>[3x]AGSFVEMVDNLRGKSGQGYYVEMTVGSPPQTLNILVDTGSSNFAVGAAPHPFLHRYYQRQLSSTYRDLRKGVYVPYTQGKWEGELGTDLVSIPHGPNVTVRANIAAITESDKFFINGSNWEGILGLAYAEIARPDDSLEPFFDSLVKQTHVPNLFSLQLCGAGFPLNQSEVLASVGGSMIIGGIDHSLYTG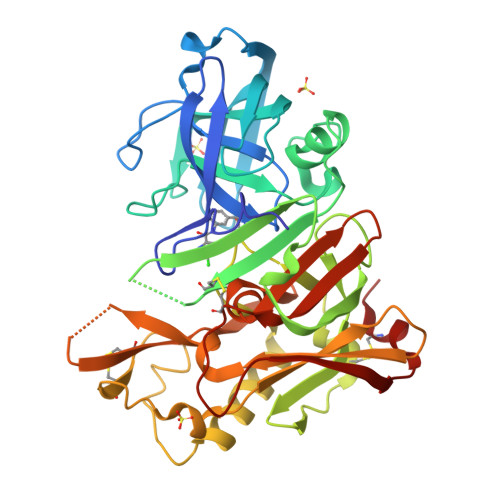SLWYTPIRREWYYEVIIVRVEINGQDLKMDCKEYNYDKSIVDSGTTNLRLPKKVFEAAVKSIKAASSTEKFPDGFWLGEQLVCWQAGTTPWNIFPVISLYLMGEVTNQSFRITILPQQYLRPVEDVATSQDDCYKFAISQSSTGTVMGAVIMEGFYVVFDRARKRIGFAVSACHVHDEFRTAAVEGPFVTLDMEDCGYN10-(3-methyl-3-oxidanyl-but-1-ynyl)-5,6-dihydroimidazo[1,2-d][1,4]benzoxazepine-2-carboxamide 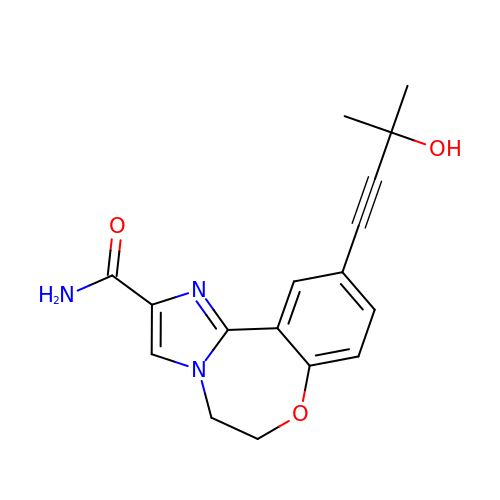| C17 H17 N3 O3 | CMHKURIYUXPNNR-UHFFFAOYSA-N> MGSSHHHHHHSSGLVPRGSHMSGVSSRPCGYWFSTNAAMTNVGEEDKQSIPSIELKENIELTDKERKIFDRLLSTLRYCNLDTQLRVAGGWVRDKLLGKESDDIDIAIDNMSGSEFLDKFKEYLSSRDEEVQGDTVIERNPDQSKHLETAKLRIYDQWIDFVNLRSEEYTENSRIPTMKFGTAKDDAFRRDLTINSLFYNINSGAVEDLTERGIDDLKSGKIVTPLPAKATFLDDPLRVLRAVRFGARFGFTLDEELKEAASSEEVRVALGEKISRERIGNEIDLMISGNGPVSAVTYLSDLKLFSVVFALPSSAEPSPPENCGSLSQSYLEAMWSLLKTPRPGKFSGEQRRLALYAAMFLPFRKTVYKDTKGKSIPVVNHIFKFSMKRKTSDAETVMNIHQTTERFRSLIPSLEVKKDVELDELTWAADILEHWKSITLNDPVIPATSKIRVLTGFLLRDIKDFWRVSLLTSLLL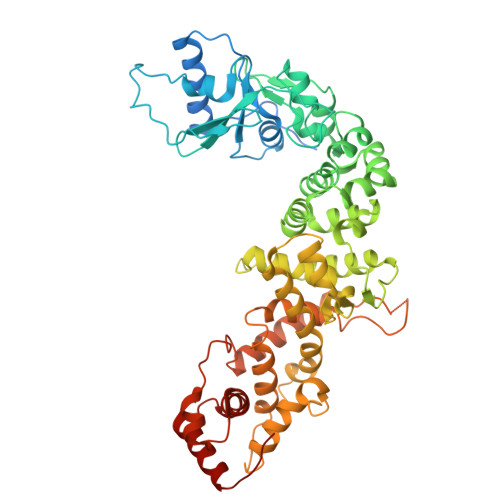SATVDGSNDHQDIGQLDFQLERMRETYLTVEATIHELGLDKIWDAKPLVNGREIMQIAELKGGSRLIREWQQKLLTWQLAYPNGTAEECKEWMRDIKAKRQRIE>GAMADREKLLTESGVYGTFATFQMDHDWWDLPGESRVISVAEVKGLVEQWSGKILVESYLLRGLSDHADLMFRVHARTLSDTQQFLSAFMGTRLGRHLTSGGLLHGVSKKPTYVAGFPESMKTELQVNGESGSRPYAIVI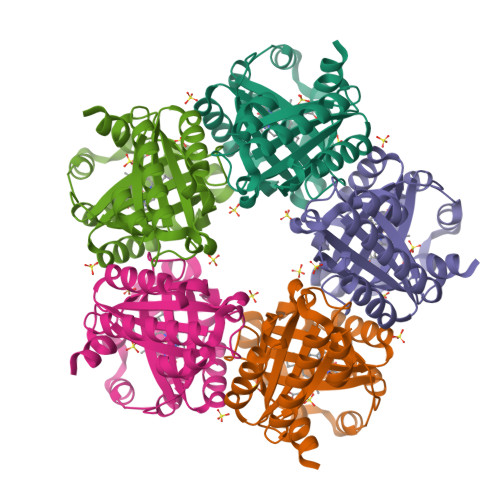PIKKDAEWWALDQEARTALMQEHTQAALPYLKTVKKKLYHSTGLDDVDFITYFETERLEDFHNLVRALQQVKEFRHNRRFGHPTLLGTMSPLDEILEKFAQ[5x]> NQIDLNVTCRYAGVFHVEKNGRYSISRTEAADLCQAFNSTLPTMDQMKLALSKGFE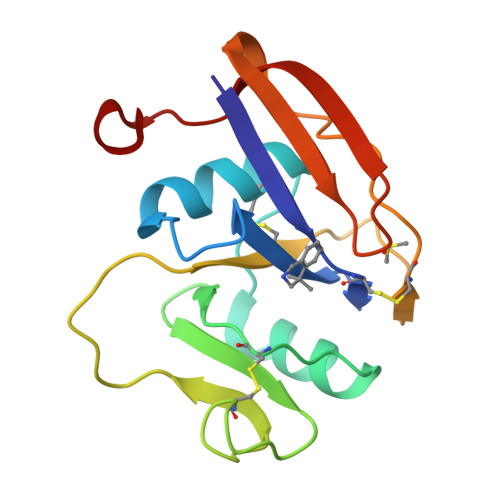TCRYGFIEGNVVIPRIHPNAICAANHTGVYILVTSNTSHYDTYCFNASAPPEEDCTSVTDLPNSFDGPVTITIVNRDGTRYSKKGEYRTHQEDID> MASQSQGIQQLLQAEKRAAEKVADARKRKARRLKQAKEEAQMEVDQYRREREQEF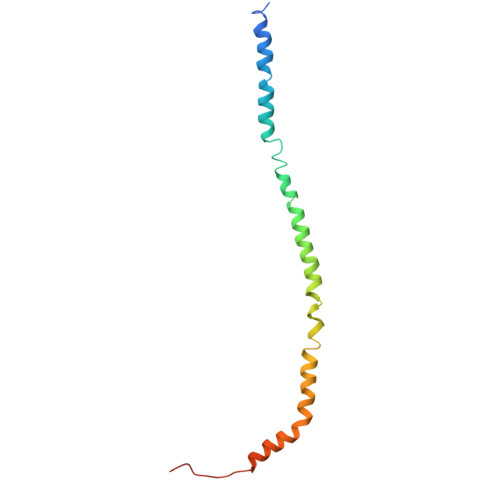QSKQQAAMGSQGNLSAEVEQATRRQVQGMQSSQQRNRERVLAQLLGMVCDVRPQVHPNYRIAA> GAGCAGACATG;> ACTCCACTCA;> CAAGT;> TCTGAGTGGTGTCTGC

In this work, we exhaustively probe the ability of all 36 immobile HJ sequences to form DNA crystals in two different designed systems. Three separate self-assembling DNA crystal systems are described in this report: the “4 × 5” and “4 × 6” designs (collectively referred to as the 4 × N systems), and a third construct with a “scrambled” sequence variant of the 4 × 6 lattices. Self-assembly was mediated by three constituent oligonucleotides: (S1) containing four sequence repeats of either 5 or 6 bases; (S2) composed of 21 bases containing complementary regions to both (S1); and (S3) which forms the second junction crossover. The HJ serves as the fundamental component at the core of each unit, and the ultimate assembly of the full lattice is facilitated by the complementary 2-base sticky ends that tail each duplex.

The 4 × 5 system robustly crystallized with 75% of the junctions, and we obtained crystals in all but 9 of 36 sequences. Of the resulting structures, 18 exhibited P32 symmetry with average cell dimensions a = b = 68.85 Å c = 60.09 Å, with only nine retaining the original P3221 symmetry with average cell edges a = b = 68.17 Å c = 60.60 Å. Although the cell parameters between the two symmetries were virtually indistinguishable, the differences between the periodicity of the lattices is dramatic, with vastly different cavity sizes. While the highest resolution achieved for the J1 system was 3.1 Å, in roughly half of the crystals measured the resolutions were 3.05 Å or better, and as high as 2.9 Å (J6) and 2.75 Å (J19), for the P32 and P3221 symmetries, respectively. Pos1 and 2 were readily observable in the electron density maps at either one or both of these conserved sites in a significant number of the structures, with no apparent respect to motif or symmetry. However, in the majority of the crystal structures reported here, the cacodylate anion indeed fits best into the electron density map of our X-ray structures, due to the presence of sodium cacodylate in the crystallization solution.> GPKGPKGPKGKPGPEGEPGEPGE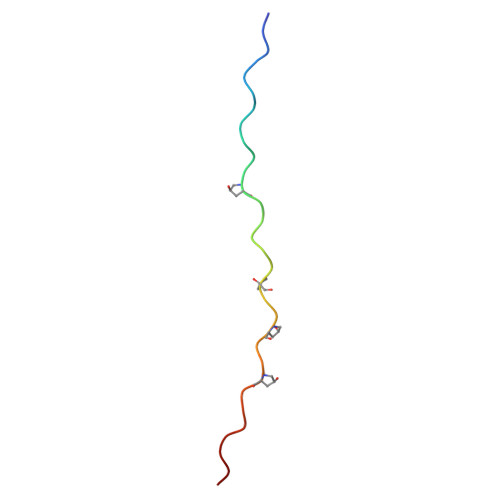PGPKGPKG> MRERLKRDLFQFNKTVEHGFPHQPSALGYSPSLRILAIGTRSGAIKLYGAPGVEFMGLHQENNAVTQIHLLPGQCQLVTLLDDNSLHLWSLKVKGGASELQEDESFTLRGPPGAAPSATQITV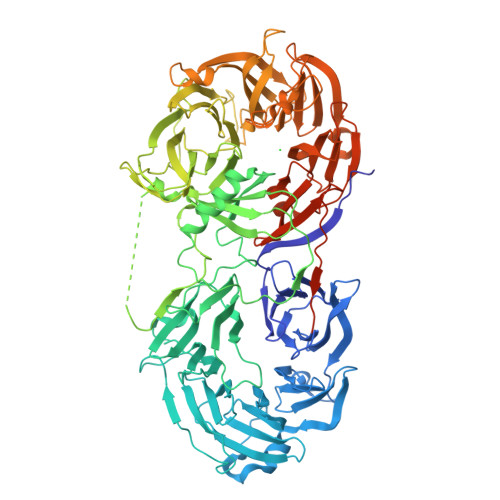VLPHSSCELLYLGTESGNVFVVQLPAFRALEDRTISSDAVLQRLPEEARHRRVFEMVEALQEHPRDPNQILIGYSRGLVVIWDLQGSRVLYHFLSSQQLENIWWQRDGRLLVSCHSDGSYCQWPVSSEAQQPEPLRSLVPYGPFPCKAITRILWLTTRQGLPFTIFQGGMPRASYGDRHCISVIHDGQQTAFDFTSRVIGFTVLTEADPAATFDDPYALVVLAEEELVVIDLQTAGWPPVQLPYLASLHCSAITCSHHVSNIPLKLWERIIAAGSRQNAHFSTMEWPIDGGTSLTPAPPQRDLLLTGHEDGTVRFWDASGVCLRLLYKLSTVRVFLTDTDPNENFSAQGEDEWPPLRKVGSFDPYSDDPRLGIQKIFLCKYSGYLAVAGTAGQVLVLELNDEAAEQAVEQVEADLLQDQEGYRWKGHERLAARSGPVRFEPGFQPFVLVQCQPPAVVTSLALHSEWRLVAFGTSHGFGLFDHQQRRQVFVKCTLHPSDQLALEGPLSRVKSLKKSLRQSFRRMRRSRVSSRKRHPAGPPGEAQEGSAKAERPGLQNMELAPVQRKIEARSAEDSFTGFVRTLYFADTYLKDSSRHCPSLWAGTNGGTIYAFSLRVPPAERRMDEPVRAEQAKEIQLMHRAPVVGILVLDGHSVPLPEPLEVAHDLSKSPDMQGSHQLLVVSEEQFKVFTLPKVSAKLKLKLTALEGSRVRRVSVAHFGSRRAEDYGEHHLAVLTNLGDIQVVSLPLLKPQVRYSCIRREDVSGIASCVFTKYGQGFYLISPSEFERFSLSTKWLVEPRCLVDSAETKNHRPGNGAGPKKAPSRARNSGTQSDGEEKQPGLVMEREFTTASENLYFQ> MNTIFSARIMKRLALTTALCTAFISAAHADDLNIKTMIPGVPQIDAESYILIDYNSGKVLAEQNADVRRDPASLTKMMTSYVIGQAMKAGKFKETDLVTIGNDAWATGNPVFKGSSLMFLKP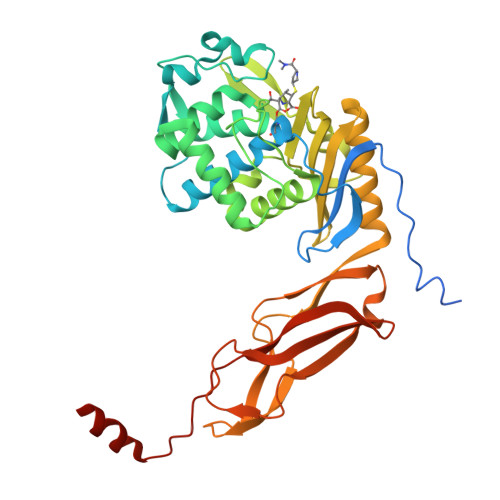GMQVPVSQLIRGINLQSGNDACVAMADFAAGSQDAFVGLMNSYVNALGLKNTHFQTVHGLDADGQYSSARDMALIGQALIRDVPNEYSIYKEKEFTFNGIRQLNRNGLLWDNSLNVDGIKTGHTDKAGYNLVASATEGQMRLISAVMGGRTFKGREAESKKLLTWGFRFFETVNPLKVGKEFASEPVWFGDSDRASLGVDKDVYLTIPRGRMKDLKASYVLNSSELHAPLQKNQVVGTINFQLDGKTIEQRPLVVLQEIPEGNFFGKIIDYIKLMFHHWFG> MEAAAGRSSHLGPAPAGRPPRCPLLLQLQLLLLLLLLPPGWVPGAAGTQGAEFPELCSYTWEAVDTKNNMLYKINICGNMGVAQCGPSSAVCMHDLKTDSFHSVGDSLLKTASRSLLEFNTTVNCKQQNHKIQSSITFLCGKTLGTPEFVTATDCVHYFEWRTTAACKKNIFKANKEVPCYAFDRELKKHDLNPLIKTSGAYLVDDSDPDTSLFINVCRDIEVLRASSPQVRVCPTGAAACLVRGDRAFDVGRPQEGLKLVSNDRLVLSYVKEGAGQPDFCDGHSPAVTITFVCPSERREGTIPKLTAKSNCRFEIEWVTEYACHRDYLESRSCSLSSAQHDVAVDLQPLSRVEASDSLFYTSEADEYTYYLSICGGSQAPICNKKDAAVCQVKKADSTQVKVAGRPQNLTLRYSDGDLTLIYFGGEECSSGFQRMSVINFECNQTAGNNGRGAPVFTGEVDCTYFFTWDTKYACVHEKEALLCGVSDGKQRFDLSALARHSELEQNWEAVDGSQREAEKKHFFINICHRVLQTGQARGCPEDAAVCAVDKNGSKNLGRFISSPTREKGNIQLSYSDGDECGGGQKIITNITLMCKPGDLESAPVLTTSRADGCFYEFEWRTAAACVLSRTEGDNCTVFDSQAGFSFDLTPLTKKDAYKVETDKYEFHINVCGPVSVGACPPDSGACQVSRSDRKSWNLGRSNAKLSYYDGMIQLTYRDGTPYNNEKRTPRATLITFLCDRDAGVGFPEYQEEDNSTYNFRWYTSYACPEEPLECIVTDPVTLDQYDLSRLAKSEGGPGGNWYSLDNGGARSTWRKYYINVCRPLNPVPGCDRYASACQMKYQGEQGSYSETVSISNLGVAKTGPMVEDSGSLLLEYVNGSACTTSDQRRTTYTTRIHLVCSTGSLYTHPIFSLNWECVVSFLWNTAAACPIRITTDIDQVCSIKDPNSGYVFDLNPLNNSRGYVVLGIGKTFLFNVCGDMPACGTLDGKPASGCEAEVQMDDMKTLKPGRLVGLEKSLQLSTEGFITLNYTGLPSHPNGRADAFIIRFVCNDDVYPGTPKFLHQDIDSSLGIRDTFFEFETALACVPSPVDCQVTDPAGNEYDLSGLSKARKPWTAVDTFDEGKKRTFYLSVCTPLPYIPGCHGTAVGCCLVTEDSKLNLGVVQISPQVGANGSLSLVYVNGDKCKNQRFSTRINLECAHTTGSPTFQLQNDCEYVFLWRTVEACPVVRAEGDYCEVRDPRHGNLYNLIPLGLNDTVVRAGEYTYYFRVCGELTSGVCPTSDKSKVISSCQEKRGPQGFQKVAGLFNQKLTYENGVLKMNYTGGDTCHKVYQRSTTIFFYCDRSTQAPVFLQETSDCSYLFEWRTQYACPPYDLTECSFKNEAGETYDLSSLSRYSDNWEAVTGTGSTEHYLINVCKSLSPQAGSDPCPPEAAVCLLGGPKPVNLGRVRDSPQWSQGLTLLKYVDGDLCPDQIRKKSTTIRFTCSESHVNSRPMFISAVEDCEYTFSWPTAAACAVKSNVHDDCQVTNPATGHLFDLSSLSGRAGFTAAYSEKGLVYLSVCGDNENCANGVGACFGQTRISVGKASKRLTYVDQVLQLVYEGGSPCPSKTGLSYKSVISFVCRPEVGPTNRPMLISLDKRTCTLFFSWHTPLACEQTTECSVRNGSSLIDLSPLIHRTGGYEAYDESEDDGSDTSPDFYINICQPLNPMHGLACPAGTAVCKVPVDGPPIDIGRVAGPPILNPIANEVYLNFESSTPCLADRHFNYTSLITFHCKRGVSMGTPKLLRTSVCDFVFEWETPLVCPDEVKTDGCSLTDEQLYYSFN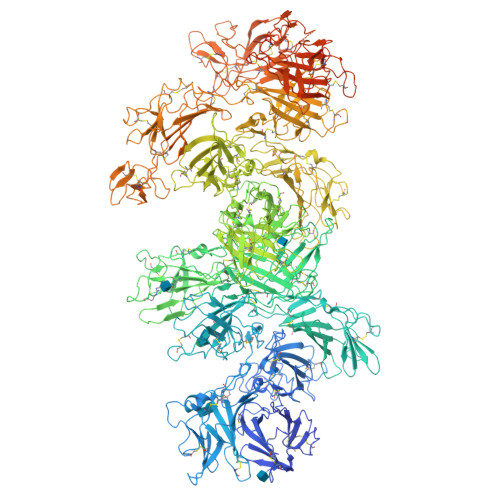LSSLSKSTFKVTRGPHTYSVGVCTAAAGLDEGGCKDGAVCLLSGSKGASFGRLASMKLDYRHQDEAVILSYANGDTCPPETEDGEPCVFPFVFNGKSYEECVVESRARLWCATTANYDRDHEWGFCKHSTSHRTSVIIFKCDEDADVGRPQVFSEVRGCEVTFEWKTKVVCPPKKMECKFVQKHRTYDLRLLSSLTGSWSFVHNGASYYINLCQKIYKGPQDCSERASVCKKSTSGEVQVLGLVHTQKLDVVDDRVIVTYSKGHYCGDNKTASAVIELTCAKTVGRPSFTRFDVDSCTYHFSWDSRAACAVKPQEVQMVNGTITNPANGRSFSLGDIYFKRFSASGDVRTNGDRYIYEIQLSSITGSSSPACSGASICQRKANDQHFSRKVGTSNQTRYYVQDGDLDVVFTSSSKCGKDKTKSVSSTIFFHCDPLVKDGIPEFSHETADCQYLFSWHTSAVCPLGAGFDEEIAGDDAQEHKGLSERSQAVGAVLSLLLVALTACLLTLLLYKKERREMVMSRLTNCCRRSANVSYKYSKVNKEEEADENETEWLMEEIQPPAPRPGKEGQENGHVAAKSVRAADTLSALHGDEQDSEDEVLTLPEVKVRPPGRAPGAEGGPPLRPLPRKAPPPLRADDRVGLVRGEPARRGRPRAAATPISTFHDDSDEDLLHV Cell division in most bacteria is regulated by the tubulin homolog FtsZ as well as ZapA, a FtsZ-associated protein. In the presence of GTP, FtsZ polymerizes into protofilaments, which further associate into a ring-like structure (the Z-ring). ZapA binds FtsZ straight protofilaments preferentially to crosslink FtsZ protofilaments; thereby, ZapA bundles more aligned and straight filaments constituting a coherent Z-ring. A FtsZ protofilament has polarity and lacks symmetry, while ZapA is in an equilibrium between homodimer and homotetramer, which are related by C2 and D2 symmetry, respectively.

In this study, we report the high-resolution cryo-EM structure of the K. pneumoniae ZapA-FtsZ complex. The cryo-EM structure of the ZapA-FtsZ complex reveals an asymmetric ladder-like architecture, in which the double antiparallel FtsZ protofilament on one side and a single protofilament on the other side are tethered by ZapA tetramers. After removing the duplicated particles, we performed helix refine with D1 symmetry, namely with a single C2 axis perpendicular to the helical axis but no rotational symmetry along the helical axis, and reached an overall map resolution of 2.73 Å with an optimized helical rise of 44.58 Å and a helical twist of −3.11°. The well-resolved FtsZ double protofilament structure enabled us to confirm that all FtsZ monomers are in the T conformation with GMPCPP bound and that the two FtsZ protofilaments are antiparallel. In the ZapA-FtsZ interface, the ZapA dimer head (chains G, H) interacted with two pairs of FtsZ dimers from two antiparallel protofilaments (chains A, B, and E, F). The N-terminal region of FtsZ (residues 1–10) was sandwiched between two ZapA molecules. The interface area of the ZapA dimer head (chains G, H) with two pairs of FtsZ dimers is extensive (2105.4 Å2) with a ΔG of dissociation of −17.0 kcal/mol, as compared with the interface area and a ΔG of dissociation between two FtsZ molecules within a FtsZ protofilament, which are 1390.6 Å2 and −16.0 kcal/mol, respectively. According to the PISA calculation, chain B and chains F and E form an interaction area of 523.4 Å2 with a ΔG of dissociation of −3.6 kcal/mol. This feature is rationalized by the electrostatic repulsions among Glu238 and Glu305 found in the inter-protofilament interactions. The entire structure of the FtsZ protofilament with ZapA was roughly similar to that without ZapA (r.m.s.d. = 1.53 Å among 918 Cα atoms for three KpFtsZ molecules within a protofilament), but ZapA binding induces structural changes in a FtsZ molecule as well as an adjacent FtsZ molecule. When comparing the structures of FtsZ within the ZapA-FtsZ complex and that of FtsZ straight protofilaments alone (PDB code: 8IBN15), approximately 2–3 Å shifts of the β2-α2 loop and the α1-β2 loop are observed (indicated by red and green arrows in Fig. 4).

>[6x]MFEPMELTNDAVIKVIGVGGGGGNAVEHMVRERIEGVEFFAVNTDAQALRKTAVGQTIQIGSGITKGLGAGANPEVGRNAADEDREALRAALDGADMVFIAAGMGGGTGTGAAPVVAEVAKDLGILTVAVVTKPFNFEGKKRMAFAEQGITELSKHVDSLITIPNDKLLKVLGRGISLLDAFGAANDVLKGAVQGIAELITRPGLMNVDFADVRTVMSEMGYAMMGSGVASGEDRAEEAAEMAISSPLLEDIDLSGARGVLVNITAGFDLRLDEFETVGNTIRAFASDNATVVIGTSLDPDMNDELRVTVVATGIGMDKRPEITLVTNKQVQQPVMDRYQQHGMSPLTQEQKPAAKVVNDNTPQTAKEPDYLDIPAFLRKQAD;>[8x]MSAQPVDLQIFGRSLRVNCPPEQRDALNQAAEDLNQRLQDLKERTRVTNTEQLVFIAALNISYELTQEKAKTRDYASSMEQRIRMLQQTIEQALLEQGRISERPGSKFE> NSSTASKTYNYVYSSDPSSLNYLAENRAATSDIVANLVDGLLENDQYGNIIPSLAEDWTVSQDGLTYTYKLRKDAKWFTSEGEEYAPVTAQDFVTGLQYAADKKSEALYLVQDSVAGLDDYITGKTSDFSTVGVKALDDQTVQYTLVKPELYWNSKTLATILFPVNADFLKSKGDDFGKADPSSILYNGPFLMKALVSKSAIEYKKNPNYWDAKNVFVDDVKLTYYDGSDQESLERNFTAGAYTTARLFPNSSSYEGIKEKYKNNIIYSMQNSTSYFFNFNLDRKSYNYTSKTSDIEKKSTQEAVLNKNFRQAINFAFDRTSYGAQSEGKEGATKILRNLVVPPNFVSIKGKDFGEVVASKMVNYGKEWQGINFADGQDPYYNPEKAKAKFAEAKKELEAKGVQFPIHLDKTVEVTDKVGIQGVSSIKQSIESVLGSDNVVIDIQQLTSDEFDSSGYFAQTAAQKDYDLYHGGWGPDYQDPSTYLDIFNTNSGGFLQNLGLEPGEANDKAKAVGLDVYTQMLEEANKEQDPAKRYEKYADIQAWLIDSSLVLPSVSRGGTPSLRRTVPFAAAYGLTGTKGVESYKYLKVQDKIVTTDEYAKAREKWLKEKEESNKKAQEELAKHVK;>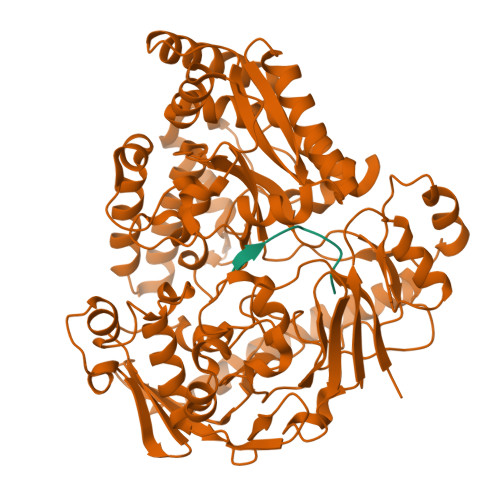 VMVKGPGPGR>QPRPAFSAIRRNPPMGGNVVIFDTVITNQEEPYQNHSGRFVCTVPGYYYFTFQVLSQWEICLSIVSSSRGQVRRSLGFCDTTNKGLFQVVSGGMVLQLQQGDQVWVEKDPKKGHIYQGSEADSVFSGFLIFPSA[2x];>[2x]ATQKIAFSATRTINVPLRRDQTIRFDHVITNMNNNYEPRSGKFTCKVPGLYYFTYHASSRGNLCVNLMRGRERAQKVVTFCDYAYNTFQVTTGGMVLKLEQGENVFLQATDKNSLLGMEGANSIFSGFLLFPDMEA;>KQKFQSVFTVTRQTHQPPAPNSLIRFNAVLTNPQGDYDTSTGKFTCKVPGLYYFVYHASHTA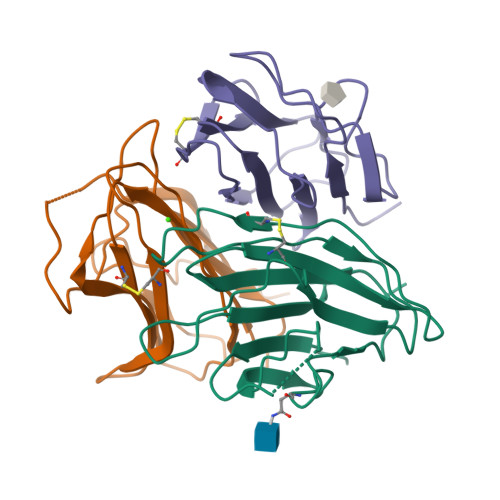NLCVLLYRSGVKVVTFCGHTSKTNQVNSGGVLLRLQVGEEVWLAVNDYYDMVGIQGSDSVFSGFLLFPD[2x]>[2x]GMTLTRDSLLTLEAYAKVR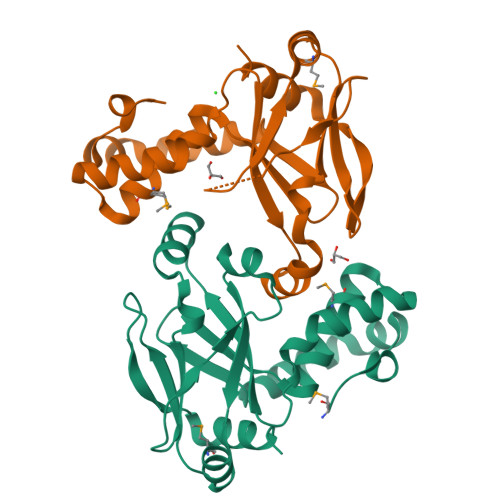RQEHARVIAHKKRRAVSIGNHLRLLFEDETTIRYQIHEMLHIEKIFDEDGIQAELDAYLPLVPDGSNLKATLQIEYENETQRRAALARLVGIEDRVFLRVDDEAPVYAIADEDLERDTAEKTSAVHFLRFELGDAMKAKLKAGAPLSIGCDHPHYPIQAARIDPDVAASLAGDLD>AQVINTFDGVADYLQTYHKLPDNYITKSEAQALGWVASKGNLADVAPGKSIGGDIFSNREGKLPGKSGRCWREADINYTSGFRNSDRILYSCDWLIYKT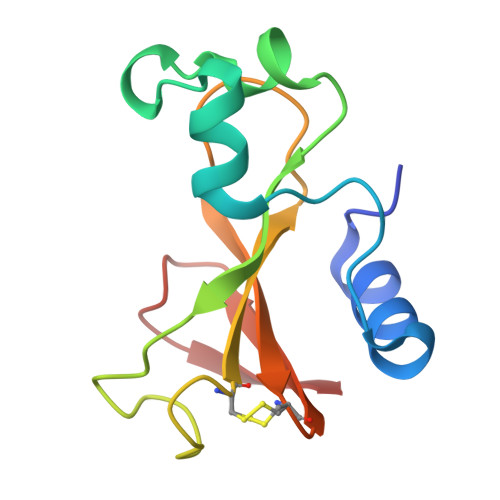TDHYQTFTKIR[3x]4'-NITROPHENYL-S-(BETA-D-GLUCOPYRANOSYL)-(1-3)-(3-THIO-BETA-D-GLUCOPYRANOSYL)-(1-3)-BETA-D-GLUCOPYRANOSIDE | C24 H35 N O17 S | 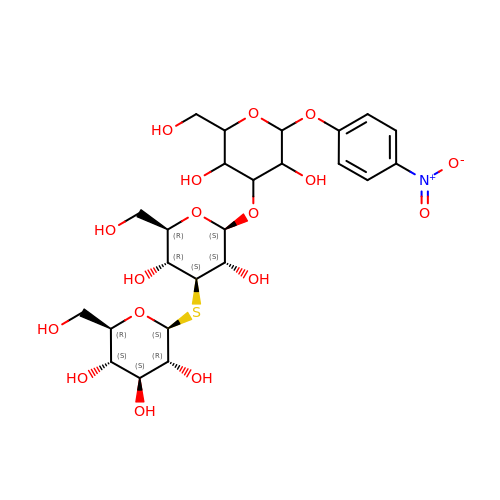VWNONHZCCMYIGR-VGNFVTAUSA-N> MAHHHHHHMEKVRVRFAPSPTGPLHLGGVRTALYDYLFAKHNGGDFILRIEDTDTQRYVPGSEEYIMEALEWIGMVPDESPKHGGPYAPYRQSERRDIYDRYTEQILKTDYAYLAFDTPEELDQIRAEFEARGDVFAYNYETRNRLRNSISLPEEEVKKLLEEKTPYVIRFKMPLDRIINLNDIIRGKFSVNTNTLDDKVLVKNDGMPTYHFANIIDDHEMKITHVIRGEEWLPSMALHVLLYEAMGWDAPEFAHLSLILKPEGKGKLSKRDGDKFGFPVFPLNFTDSATGNTSAGYREEGYLPEAFINMVAMLGWSPADNKEIVSMDEMIKEFDLNKVHKAGARFSAEKAKWFNQQYLQLMSNEAILPEFKKVLAENNVEVSDEKALKIIGLMKERATFVKDIYNDGKFFFHAPESFDEKASKKAWSPETAVLMQELTEAISSLDFKAEIIKESIHHLAEAKGLGMGKVMMPLRLSLVGELKGPDVPDLMEMIGKEETISRINKAIETLK

Glutamyl-tRNA synthetase (GluRS) is essential for tRNA aminoacylation and is under investigation as a bacterial drug target. GluRS catalyzes tRNA aminoacylation: the binding of glutamate to tRNA. The structures of Elizabethkingia GluRSs reported here share ∼97% sequence identity. EmGluRS and EaGluRS are monomeric enzymes that assemble with a prototypical GluRS topology with an N-terminal tRNA synthetase class I (E and Q) catalytic domain and a C-terminal anticodon-binding domain.

EmGluRS was co-crystallized with glutamate, while EaGluRS is an apo structure. EmGluRS shares ∼97% sequence identity with EaGluRS but less than 39% sequence identity with any other structure in the Protein Data Bank. The EmGluRS and EaGluRS structures are very similar and have a root-mean-squared difference of ∼1.3 Å for the alignment of all main-chain Cα atoms. ENDScript analyses revealed that despite having <40% sequence similarity, EmGluRS and EaGluRS share significant secondary-structural similarity with other bacterial GluRSs and other aminoacyl-tRNA synthetases, including some that have shown promise as drug targets. The N-terminal tRNA synthetase binding domains of all of these proteins have a sizeable accessible glutamate-binding site that is evident in the surface plot. Intriguingly, the glutamate-binding cavity has been probed to develop promising inhibitors for Pseudomonas aeruginosa GluRS (PaGluRS; Hu et al., 2015).> MSAPTDDTPTDAIAAPRHSAPPRPRLPWFLRTFAVPIILAWVAVVAILNTVVPTLDEVGEMRAVSMAPNDAPSTLAIKRVGQVFEEYDTSSSVMIVLEGEEPLGIEAHAFYDKMVADLRADTEHVQHVQDFWGDTLTASGAQSVDGKAAYVQVYIAGDQGESLANESVEAVRKIATERETPSGVKAYVTGAAATSADQRAEGDASMKLIEGVTFAVITVMLLAVYRSVITTLIVLAMVVLGLSGARGIVAFLGFYNVFGLTTFATNMVVTLAIAAATDYAIFLIGRYQEARRAGEDRESAYYTMFHGTAHVVLASGLTIAGATLCLHFTRLPYFQTMGVPLAIGMLIVVAAALTAGPAVISVVSRFGKTLEPKRFSRSPGWHRVGTATVRWPGAILVCAVVAALIGLLALPGYYTTYDDRRYLPDDVPANVGYDAAFRHFSQAKMNPDLMMVETDRDLRNPADFLVIDKIAKALKNVHGIAQVQTITRPDGDPIEHSTIPYTIGQSGTTQIMNNDYMQTNLDNLLKQADDLQTSIDSMTEMMNIQTELAAVSQSMADKMAQTSDDTADVRDHLADFDDFFRPIRNYLYWEPHCYDIPMCWSMRSIFESIDGINTMSDDFQELVPEMRRMADLMPRMVAVMPAQIQSMKNQKQTLLNQYQVQKAQQDQNMAMQENATAMSQAFDAAKNDDSFYLPPEAFETDDFQRGMKLFMSPDGHAVRFTIIHQGDPLTEEGTARMDELKVAAADAIKGTPFEGARIYLGGSAATYNDMQIGADYDLIIVAASALILIFIIMMVLTRAVVAAAVIVGTVVLSLASAFGLSVLLWQHIVGIPLHWMVLPMSVIVLLAVGADYNLLLVSRMKEEIHAGIRTGIIRAMVGTGAVVTAAGLVFAFTMASMAVSSLITIGQVGTTIGLGLLFDTLVVRSLMTPSIATLLGRWFWWPQRVRERPVPSKWPTPIQRTPEEALSHHHHHH

The genome of Mtb encodes 13 mycobacterial membrane protein large (MmpL) transporters. These membrane proteins belong to a subfamily of the resistance-nodulation cell division (RND) superfamily of transporters and are critical for mycobacterial physiology and pathogenesis, with several of these transporters involved in the export of fatty acids and lipid components to the cell envelope. MmpL4 and MmpL5 share similar functions in siderophore export and are required for iron acquisition. Mycobacteria secrete mycobactin (Mbt) and carboxymycobactin (Cmb), siderophores with an extremely high affinity for Fe(III), via the MmpL4 and MmpL5 transporters to recruit this important metal that is essential for growth and survival. According to the protein sequence alignment with MmpL3, it is speculated that both MmpL4 and MmpL5 are proton motive force (PMF)-dependent transporters that function via a proton/substrate antiport mechanism.

The cryo-EM structure of MmpL5 embedded in LMNG detergent micelles was solved to a nominal resolution of 3.00 Å. The cryo-EM structure of MmpL5 is nearly identical to that of MmpL4. Superimposition of these 2 structures gives rise to an RMSD of 0.9 Å (for 681 Cα atoms). However, cryo-EM densities for the majority of residues making up the periplasmic subdomain PD3 are missing, similar to what was seen with MmpL4. Distinct from MmpL4, the structure of MmpL5 indicates that this transporter only possesses one channel that spans the outer leaflet of the transmembrane domain up through the periplasmic domain. However, the midway point of this channel is much narrower, suggesting that the structure of MmpL5 may depict a different intermediate state with respect to that of MmpL4. In MmpL5, the section of TM8 located at the outermost surface of the cytoplasmic membrane shifts into the core of the membrane protein by as much as 3.5 Å in relation to the position of TM8 in MmpL4. In MmpL5, the narrowest region of the channel is surrounded by residues Y417, Y767, Q771, and W835, residues that may be important for controlling the width of the MmpL5 channel. Similar to MmpL4, residue D278 and Y852 of MmpL5 interact with each other and create a hydrogen bond, presumably relaying protons for energy coupling. Autodock Vina suggests that MmpL5 binds Mbt in the transmembrane pocket and periplasmic cavity with affinities of −7.9 and −8.0 kcal/mol, which correspond to KDs of 1.6 and 1.3 μm, respectively.> GPHMATGQDRVVALVDMDCFFVQVEQRQNPHLRNKPCAVVAYKSWKGGGIIAVSYEARAFGVTASMWADDAKKLCPDLLLAQVRESRGKANLTKYREASVEVMEIMS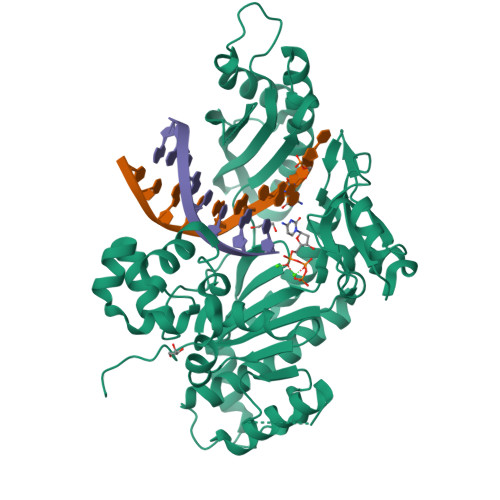RFAVIERASIDEAYVDLTSAVQERLQKLQGQPISADLLPSTYIEGLPQGPTTAEETVQKEGMRKQGLFQWLDSLQIDNLTSPDLQLTVGAVIVEEMRAAIERETGFQCSAGISHNKVLAKLACGLNKPNRQTLVSHGSVPQLFSQMPIRKIRSLGGKLGASVIEILGIEYMGELTQFTESQLQSHFGEKNGSWLYAMCRGIEHDPVKPRQLPKTIGCSKNFPGKTALATREQVQWWLLQLAQELEERLTKDRNDNDRVATQLVVSIRVQGDKRLSSLRRCCALTRYDAHKMSHDAFTVIKNCNTSGIQTEWSPPLTMLFLCATKFSAS> MASMERFLSVYDEVQAFLLDQLQSKYEIDPNRARYLRIMMDTTCLGGKYFRGMTVVNVAEGFLAVTQHDEATKERILHDACVGGWMIEFLQAHYLVEDDIMDGSVMRRGKPCWYRFPGVTTQCAINDGIILKSWTQIMAWHYFADRPFLKDLLCLFQKVDYATAVGQMYDVTSMCDSNKLDPEVAQPMTTDFAEFTPAIYKRIVKYKTTFYTYLLPLVMGLFVSEAAASVEMNLVERVAHLIGEYFQVQDDVMDCFTPPEQLGKVGTDIEDAKCSWLAVTFLGKANAAQVAEFKANYGDKDPAKVAVVKRLYSEANLQADFAAYEAEVVREVESLIEQLKVKSPTFAESVAVVWEKTHKR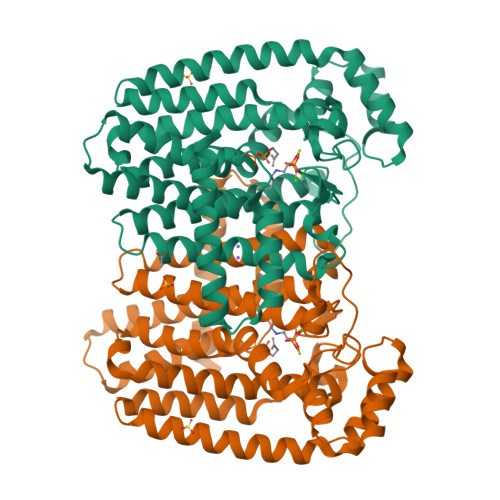KK Most eukaryotes have two Rad51/RecA recombinases: Rad51, which is expressed constitutively, and Dmc1, which is only expressed in meiosis. Rad51 and Dmc1 are both ATP-dependent DNA-binding proteins and both form extended helical filaments on ssDNA, which are key intermediates in HR. ATP binding promotes filament assembly, whereas the hydrolysis of ATP to ADP reduces filament stability to promote filament disassembly. Here, we present cryo-EM structures of S. cerevisiae Rad51 and Dmc1 nucleoprotein filaments in their ADP-bound states.

To solve the cryo-EM structures of S. cerevisiae Rad51 and Dmc1 in the ADP-bound states, we mixed the purified proteins with 96-nucleotide ssDNA oligonucleotide in the presence of 2 mM ADP. Interestingly, in contrast to our observations with Rad51, the Dmc1 filaments were interdigitated, similar to what was recently observed for human RAD51 filaments in the presence of ADP. At this time, we do not have any reason to believe that these interdigitated structures reflect a biologically meaningful intermediate. Therefore, the interdigitated filaments were computationally deconvolved into single helical filaments, yielding well-defined structures with an overall resolution of 2.7 Å. In the Dmc1 ADP-bound structure, the helical pitch increased to 133 Å, corresponding to an overall increase in the contour length of 35.2%, there were 6.6 monomers per turn and each protomer was rotated 47.4° relative to its neighbors, and the filament had a maximum width of 97.5 Å. Previous studies have shown, mutation of H352 within S. cerevisiae Rad51 to alanine, tyrosine, phenylalanine, lysine, or methionine, severely compromises both ATP hydrolysis activity and nucleoprotein filament assembly at physiological pH. Consistent with this model, we find that Rad51 H352 and Dmc1 H289 move away from the neighboring protomers when the nucleoprotein filaments are in the ADP-bound states, corresponding to a shift of 4.8 Å in the case of Rad51 and 5.3 Å for Dmc1 measured from the epsilon carbon if the histidine side chains. Comparison of the ATP-bound and ADP-bound states reveals that S. cerevisiae Rad51 D374 and Dmc1 D311 move away from the neighboring protomer in the ADP-bound states, corresponding to a distance (measured from the alpha carbon) of 2.7 Å in the case of Rad51 and 3.7 Å for Dmc1. For Dmc1, residues F244, R248, and E251 interact with V224 and R187 from the adjacent protomer in the ATP-bound state. Lastly, similar to Rad51, Dmc1 residue R52 from one protomer contacts residue E231 in the L1 DNA-binding loop of the adjacent protomer. As with Rad51, all of these contacts are disrupted in the ADP-bound state of Dmc1.

>[6x]MSVTGTEIDSDTAKNILSVDELQNYGINASDLQKLKSGGIYTVNTVLSTTRRHLCKIKGLSEVKVEKIKEAAGKIIQVGFIPATVQLDIRQRVYSLSTGSKQLDSILGGGIMTMSITEVFGEFRCGKTQMSHTLCVTTQLPREMGGGEGKVAYIDTEGTFRPERIKQIAEGYELDPESCLANVSYARALNSEHQMELVEQLGEELSSGDYRLIVVDSIMANFRVDYCGRGELSERQQKLNQHLFKLNRLAEEFNVAVFLTNQVQSDPGASALFASADGRKPIGGHVLAHASATRILLRKGRGDERVAKLQDSPDMPEKECVYVIGEKGITDSSD> M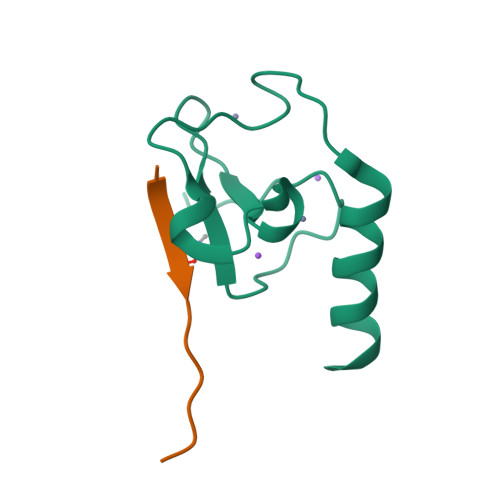GIITCICDLNDDDGFTIQCDHCNRWQHAICYGIKDIGMAPDDYLCNSCDPREVDINLARKIQQERINVK;> ARTKQTARKST The FliPQR complex forms a channel for export of flagellar structural subunits. It also acts as a template for FliE assembly within the Membrane-supramembrane-ring. Five FliP subunits and one FliR subunit assemble into a right-handed helical structure with a narrow central pore. Four FliQ subunits peripherally associate on the outside of the FliP5–FliR1 complex.

To address this issue, we conducted cryoelectron microscopy (cryoEM) structural analysis of the purified Salmonella FliPQR complex reconstituted in a peptidisc, which is a sheet of short amphipathic bihelical peptides, and obtained the structure of the completely closed form at 3.0 Å resolution. After iterative 3D refinement with C1 symmetry, the 3D image of the FliPQR complex was reconstructed at 3.0 Å resolution from 109,333 particles (EMDB ID: EMD-61993). In agreement with previous reports, the FliPQR complex adopts a right-handed helical structure composed of 5 FliP subunits, 4 FliQ subunits, and 1 FliR subunit. The densities corresponding to residues 22 to 41 of four mature FliP subunits, FliP2, FliP3, FliP4, and FliP5, and residues 1 to 5 of FliR are clearly visible, enabling us to build the atomic model of these N-terminal regions. The N-terminal region of the four FliP subunits whose N termini are resolved forms a β-hairpin with β-strands β1 and β2. The N-terminal region of FliR contains a single β-strand (β1). These β-strands form a β-sheet at the tip of the FliPQR complex, which we named the β-cap. A total of six tryptophan residues, five Trp-38 of FliP and Trp-9 of FliR, stabilize the β-cap structure via hydrophobic contacts with each other. Furthermore, the N-terminal α-helix (α1) of FliP1 projects toward the export channel, and its N-terminal region, including Trp-38, inserts into the cavity of the β-cap, thereby maintaining the closed state of the periplasmic gate. The β-cap has a narrow pore between FliP5 and FliR that is wide enough to allow the passage of a single α-helix (Left).

>MRRLLFLSLAGLWLFSPAAAAQLPGLISQPLAGGGQSWSLSVQTLVFITSLTFLPAILLMMTSFTRIIIVFGLLRNALGTPSAPPNQVLLGLALFLTFFIMSPVIDKIYVDAYQPFSEQKISMQEALDKGAQPLRAFMLRQTREADLALFARLANSGPLQGPEAVPMRILLPAYVTSELKTAFQIGFTIFIPFLIIDLVIASVLMALGMMMVPPATIALPFKLMLFVLVDGWQLLMGSLAQSFYS[5x];> MIQVTSEQWLYWLHLYFWPLLRVLALISTAPILSERAIPKRVKLGLGIMITLVIAPSLPANDTPLFSIAALWLAMQQILIGIALGFTMQFAFAAVRTAGEFIGLQMGLSFATFVDPGSHLNMPVLARIMDMLAMLLFLTFNGHLWLISLLVDTFHTLPIGSNPVNSNAFMALARAGGLIFLNGLMLALPVITLLLTLNLALGLLNRMAPQLSIFVIGFPLTLTVGIMLMAALMPLIAPFCEHLFSEIFNLLADIVSEMPINNNPHHHHHHHHHH;>[4x]MTPESVMMMGTEAMKVALALAAPLLLVALITGLIISILQAATQINEMTLSFIPKIVAVFIAIIVAGPWMLNLLLDYVRTLFSNLPYIIG isoquinoline-1,3,4(2H)-trione | C9 H5 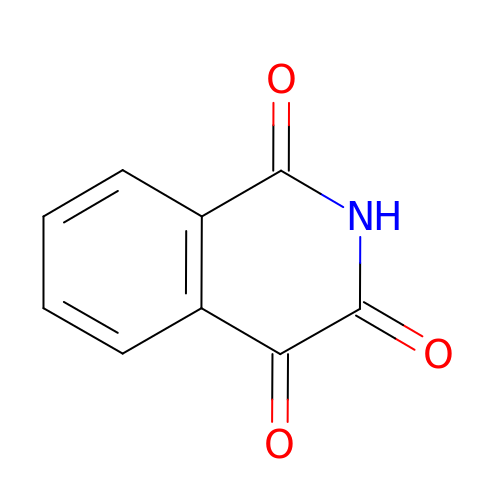N O3 | YIOFGHHAURBGSJ-UHFFFAOYSA-N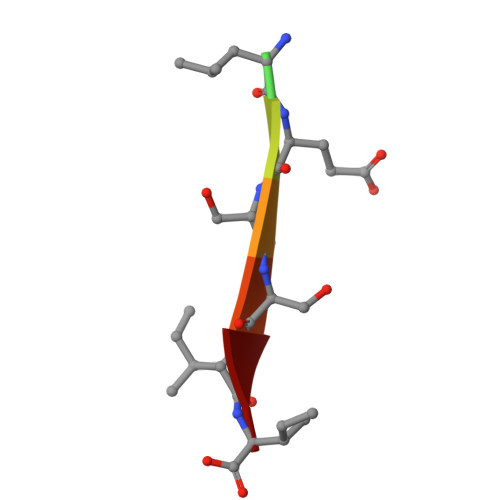> LRLESSII The heterotrimeric RNA-dependent RNA polymerase (RdRp) of influenza virus is composed of subunits PA, PB1 and PB2. It is responsible for replication and transcription of the segmented, single-stranded viral RNA genome (vRNA) in the nucleus of infected cells. Transcription of viral mRNAs occurs through a unique “cap-snatching” mechanism. We initially screened metal-chelating compounds by CEN enzymatic assays, followed by a cellular phenotypic screen and then optimized the chemical structure to improve the pharmacokinetics and safety. This culminated in the generation of the compounds BXA and BXM that target the CEN in the PA proteins of influenza A and B viruses.

All four PA-BXA co-crystal structures exhibit clear and unambiguous electron density for the compound, which is bound in essentially the identical fashion in each structure. When this residue is mutated to the more polar threonine, the structure is essentially unchanged in both the FluA and FluB structures except for the side-chain of the residue. The side-chain of T38 is orientated such that its methyl-group is in exactly the same position as the CG1 of Ile38, whereas the OH group is orientated towards helix α3 allowing it to make two hydrogen bonds to the main-chain carbonyl oxygens of Met34 and Leu35. Thus, substitution of Ile38 by Thr38 reduces slightly the van der Waals interaction with the compound since threonine lacks the CD1 methyl group of isoleucine. Furthermore, unlike I38, which does not change conformation upon BXA binding, T38 (and M34 in the case of FluB) have to change rotamer to accommodate the inhibitor binding. These two effects (less favourable van der Waals packing and induced fit change of threonine rotamer) plausibly account for the reduced affinity of the inhibitor for the I38T variant and hence the lower susceptibility of viruses bearing this mutation. The reduction of susceptibility to BXM for the I38T mutant is less for FluB compared to FluA. Since the direct effect of the substitution, as observed in the crystal structures, is essentially the same in FluA and FluB this suggests that the contribution of I38 to the affinity of the compound is proportionally less in FluB than in FluA.

> GAMGSGMAMDTFITRNFQTTIIQKAKNTMAEFSEDPELQPAMLFNTCVHLEVCYVISDMNFLDEEGKSYTALEGQGKEQNLRPQYEVIEGMPRTIAWMVQRSLAQEHGIETPKYLADLFDYKTKRFIEVGITKGLADDYFWKKKEKLGNSMELMIFSYNQDYSLSNESSLDEEGKGRVLSRLTELQAELSLKNLWQVLIGEEDVE> MGQTATTVPEFPSKLDWLNTAPLQFRRDLKGKVVILDFWTYSSINSMHVLPD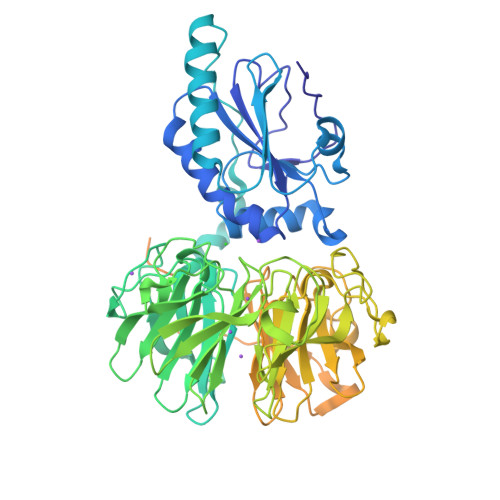LEFLEKKYKDMPFTVVGVHSAKFDNEKDLDAIRNAVLRYDISHPVVNDGDMYMWRELGINSWPTFAVVSPNGKVIAQIAGEGHRKDLDDVVAAALTYYGGKNVLDSTPLPTRLEKDNDPRLATSPLKFPGKLAIDTLNNRLFISDSNHNRIIVTDLEGNFIVQIGSSGEEGFQDGSFEDAAFNRPQGLAYNAKKNLLYVADTENHALREIDFVNERVQTLAGNGTKGSDYQGGRKGTKQLLNSPWDVCFEPVNEKVYIAMAGQHQIWEYSVLDGITRVFSGNGYERNLNGSTPQTTSFAQPSGISLGPDLKEAYIADSESSSIRALDLQTGGSRLLAGGDPYFSENLFKFGDNDGVGAEVLLQHPLGVLCANDGQIYLTDSYNHKIKKLDPVTKRVVTLAGTGKAGFKDGKVKGAQLSEPAGLAITENGRLFVADTNNSLIRYIDLNKGEDSEILTLELKGVQPPTPKAKSLKRLRKRASADTKIVKVDSVTSREGDLNLKISLPDGYHFSKEARSKFVVDVEPENAVAIDPTEGTLSPEGSTMLHFIQSSTSASVGKISCKVYYCKEDEVCLYQSVQFEVPFKVESELSASPTITFTVTPRAPDAGGLQLQGTR> MPVKLAQALANPLFPALDSALRSGRHIGLDELDNHAFLMDFQEYLEEFYARYNVELIRAPEGFFYLRPRSTTLIPRSVLSELDMMVGKILCYLYLSPERLANEGIFTQQELYDELLTLADEAKLLKLVNNRSTGSDVDRQKLQEKVRSSLNRLRRLGMVWFMGHDSSKFRITESVFRFGADVRAGD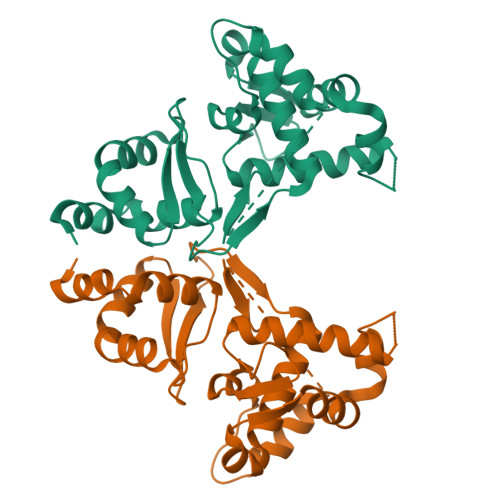DPREAQRRLIRDGEAMPIENHLQLNDETEESQPDSGEEE> GPMTTTERPDLAWLDEVTMTQLERNPYEVYERLRAEAPLAF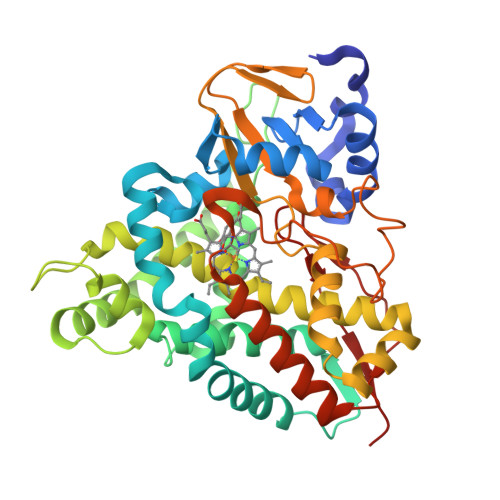VPVLGSYVASTAEVCREVATSPDFEAVITPAGGRTFGHPAIIGVNGDIHADLRSMVEPALQPAEVDRWIDDLVRPIARRYLERFENDGHAELVAQYCEPVSVRSLGDLLGLQEVDSDKLREWFAKLNRSFTNAAVDENGEFANPEGFAEGDQAKAEIRAVVDPLIDKWIEHPDDSAISHWLHDGMPPGQTRDREYIYPTIYVYLLGAMQEPGHGMASTLVGLFSRPEQLEEVVDDPTLIPRAIAEGLRWTSPIWSAGARISTKPVTIAGVDLPAGTPVMLSYGSANHDTGKYEAPSQYDLHRPPLPHLAFGAGNHACAGIYFANHVMRIALEELFEAIPNLERDTREGVEFWGWGFRGPTSLHVTWEV> SLPSFIEHSSFGVKESNPYNKLFEERIIFLGVQVDDASANDIMAQLLVLESLDPDRDITMYINSPGGGFTSLMAIYDTMQYVRADIQTVCLGQAASAAA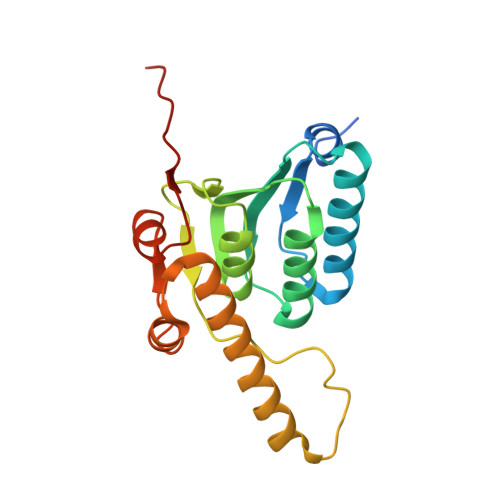VLLAAGTPGKRMALPNARVLIHQPSLSGVIQGQFSDLEIQAAEIERMRTLMETTLARHTGKDAGVIRKDTDRDKILTAEEAKDYGIIDTVLEYRKLSAQTA>[6x]MPTPNPLPVKGAGTTLWVYKGNGDPYANPLSDVDWSRLAKVKDLTPGELTAESYDDSYLDDEDADWTATGQGQKSAGDTSFTLAWMPGEQGQQALLAWFNEGDTRAYKIRFPNGTVDVFR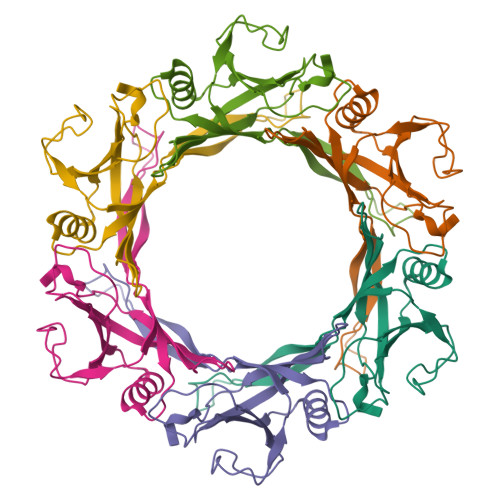GWVSSIGKAVTAKEVITRTVKVTNVGRPSMAEDRSTVTAATGMTVTPASASVVKGQSTTLTVAFQPEGATDKSFRAVSSDKTKATVSVSGMTITVNGVAAGKVNIPVVSGNGEFAAVAEITVTAS> QVEVVTQDERKALHTTASLRCSLKTSQEPLIVTWQKKKAVSPENMVTYSKTHGVVIQPAYKDRINVTELGLWNSSITFWNTTLEDEGCYMCLFNTFGSQKVSGTACLTLYV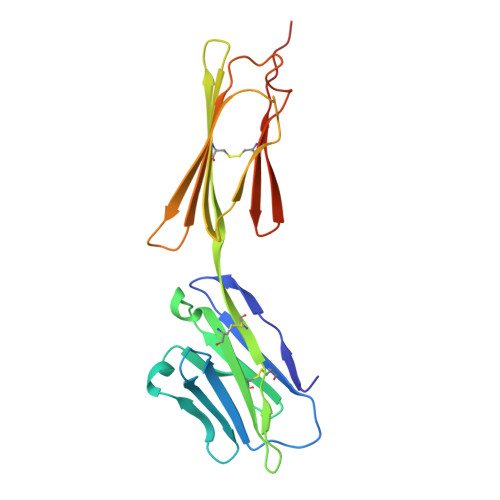QPIVHLHYNYFEDHLNITCSATARPAPAISWKGTGTGIENSTESHFHSNGTTSVTSILRVKDPKTQVGKEVICQVLYLGNVIDYKQSLDKGSTRHHHHHH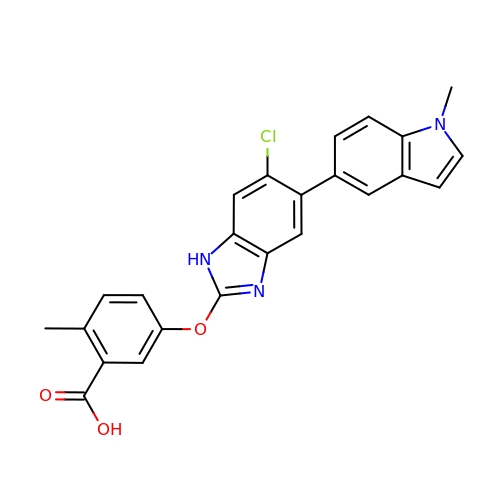5-[[6-chloranyl-5-(1-methylindol-5-yl)-1H-benzimidazol-2-yl]oxy]-2-methyl-benzoic acid | C24 H18 Cl N3 O3 | FHWSAZXFPUMKFL-UHFFFAOYSA-N>[2x]MMTRSGHPVTLDDLPLRADLRGKAPYGAPQLAVPVRLNTNENPHPPTRALVDDVVRSVREAAIDLHRYPDRDAVALRADLAGYLTAQTGIQLGVENIWAANGSNEILQQLLQAFGGPGRSAIGFVPSYSMHPIISDGTHTEWIEASRANDFGLDVDVAVAAVVDRKPDVVFIASPNNPSGQSVSLPDLCKLLDVAPGIAIVDEAYGEFSS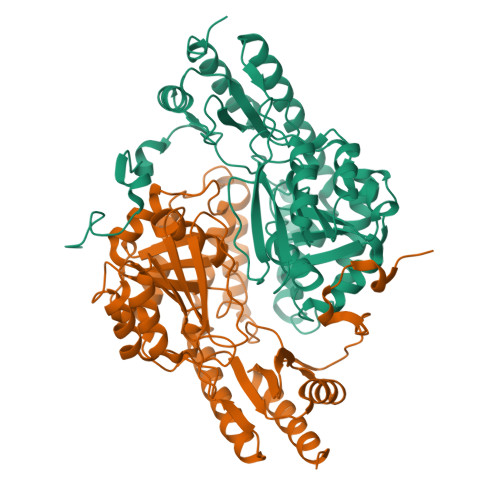QPSAVSLVEEYPSKLVVTRTMSKAFAFAGGRLGYLIATPAVIDAMLLVRLPYHLSSVTQAAARAALRHSDDTLSSVAALIAERERVTTSLNDMGFRVIPSDANFVLFGEFADAPAAWRRYLEAGILIRDVGIPGYLRATTGLAEENDAFLRASARIATDLVPVTRSPVGAPKLAAALEHHHHHH>MALLKRVVSEVVATFLLVFMTAGAAGISGSDLSRISQLGQSIAGGLIVVVMIYAVGHISGAHMNPAVTLAFAVFRHFPWIQVPFYWAAQFTGAIAASFVLKAVIHPVDVIGTTTPVGPHWHSLVVEVIVTFNMMFVTLAVATDTRAVGELAGLAVGSAVCITSIFAGAISGGSMNPARTLGPALASNRFDGLWIYFLGPVMGTLSGAWVYTFIRFEDTPREGSSQKLSSFKLRRLRSQQSIAADDVDEMENIQV[8x]

Silicon (Si), the most abundant mineral element in the earth’s crust, is taken up by plant roots in the form of silicic acid through Low silicon rice 1 (Lsi1). Lsi1 belongs to the Nodulin 26-like intrinsic protein subfamily in aquaporin and shows high selectivity for silicic acid. High accumulation of Si in rice shoots is achieved by the cooperation of two different transporters for silicic acid; Low Si rice 1 and 2 (Lsi1 and Lsi2). Lsi1 belongs to the Nodulin 26-like intrinsic proteins (NIPs) subfamily in the aquaporin (AQP) family, while Lsi2 belongs to the ion transporter superfamily.

However, we failed to obtain crystals of full-length Lsi1, so we screened a large variety of mutant Lsi1 and found that a mutant starting at Leu47 and ending at Arg264 (ΔN44/ΔC24/K50R/C66A/T93V/C139A/K232R/T253V/K264R) gave rise to crystals. This Lsi1 variant, Lsi1cryst, is functional in transporting Ge (Si analog) based on assay in Sf9 insect cells. We corrected X-ray intensities with the approach of Wang et al. and solved the structure of Lsi1cryst at 1.8 Å resolution. The structure of Lsi1cryst reveals a tetrameric fold similar to other AQPs from bacteria, plants, and animals. The structure reveals transmembrane helical orientations different from other aquaporins, characterized by a unique, widely opened, and hydrophilic selectivity filter (SF) composed of five residues. SF of AQP1 is narrower and hydrophilic (Phe58TM2/His182TM5/Cys191LE1/Arg197LE2), and that of GlpF is wider and amphipathic (Trp48TM2/Gly191TM5/Phe200LE1/Arg206LE2), whereas that of Lsi1cryst is the widest and hydrophilic (Thr65TM1/Gly88TM2/Ser207TM5/Gly216LE1/Arg222LE2). The most striking feature of the Lsi1cryst’s SF arises from an additional “fifth residue” Thr65 in TM1 (Thr65TM1) and a water molecule hydrogen-bonded to Thr65TM1 (Wat9). In Lsi1cryst, however, Gly88TM2 exposes Thr65TM1 to the channel, thereby making SF wide and hydrophilic. A striking feature of the channel of Lsi1cryst is that a large number of water molecules at the extracellular half of the pore are not in a single file, which is brought by the hydrophilic SF in the broad channel. Therefore, unlike other AQPs, the channel of Lsi1cryst has two polar faces.>SAPANAVAADDATAIALKYNQDATKSERVA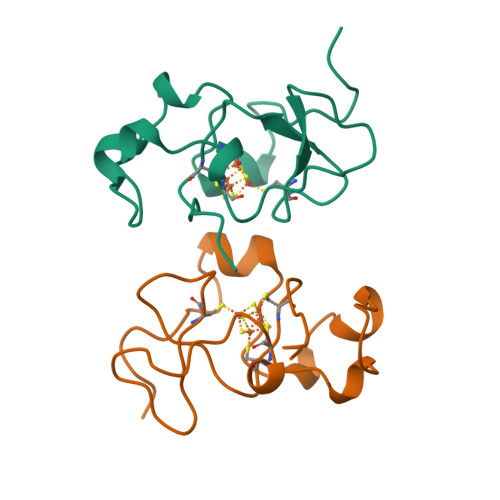AARPGLPPEEQHCANCQFMQADAAGATDEWKGCQLFPGKLINVNGWCASWTLKAG[2x]1-(3,4-dichlorobenzyl)-3,7-dimethyl-8-morpholin-4-yl-3,7-dihydro-1H-purine-2,6-dione 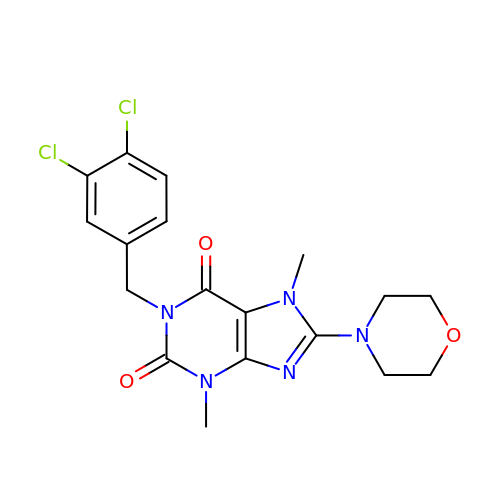| C18 H19 Cl2 N5 O3 | BFRVAZYYGGLHQS-UHFFFAOYSA-N>MHHHHHHENLYFQGAGAGAGAGAMSELSAIETAAAIAGGSMTALEACDAAIARIEQRDGPINAVVVRDFDRARDAAKAADAEIAAAVRKPLLGVPMTIKESFDIAGLPTSWGFAEHADHIATADSLVVSRLKAAGAVFLGKSNIPVGLADWQSVNPNYGRTNNPHDHSRSAGGSSGGAAAALAAGMVPLEYGSDIGGSIRVPAHFCGVWGLKTTFDAVSLEGHYFPRTDSAKADLSVVGPMARTPADLALALDITSKVPLPQSRIANLSGLRILLLTAHPETVADSATISAVERAAAACEASGATVATSSPDLPDLSALVADYTRMLLVVLARGLAPEGTEPVSLNAWYAMLD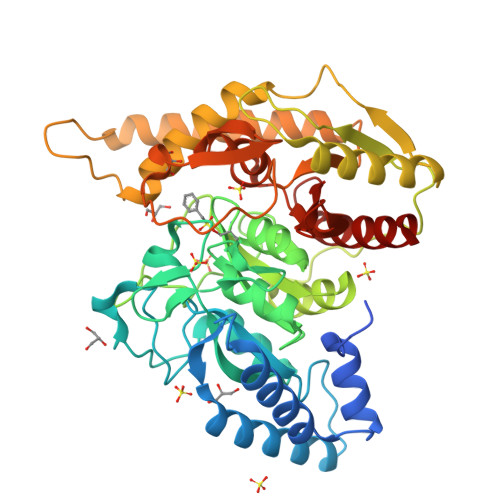DQARMMRAFDRLFESFDAIFCPVLGTTAFAHSDEPDWAKRSLSIDGGIAPFAAQLGWISMATYGGMPALSMPLGADGNGLPINLQIITRNWSDHDAIRIGALVAEALDR[2x]>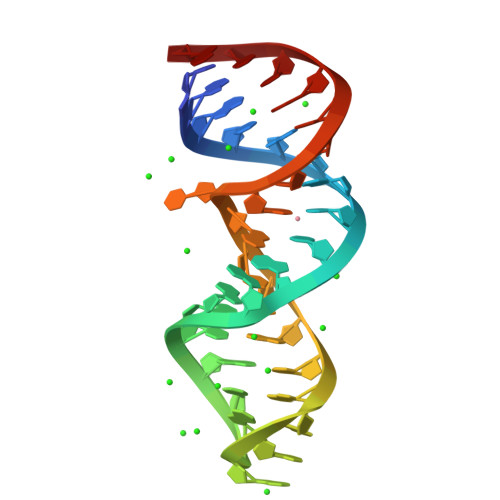 CAGCAGGCUAAGGCAUGAAAGTGCTATGCCTGCTG>[2x]MSYQS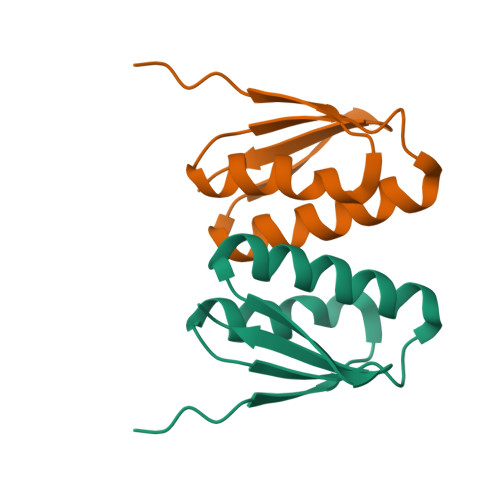TIVPVELHSFEDAQVIGGAFRDGDAVVFDMSLLSREEARRIVDFAAGLCFALRGKMQKIDSVTFAVVPE4'-(4-aminobenzoyl)biphenyl-4-sulfonamide | C19 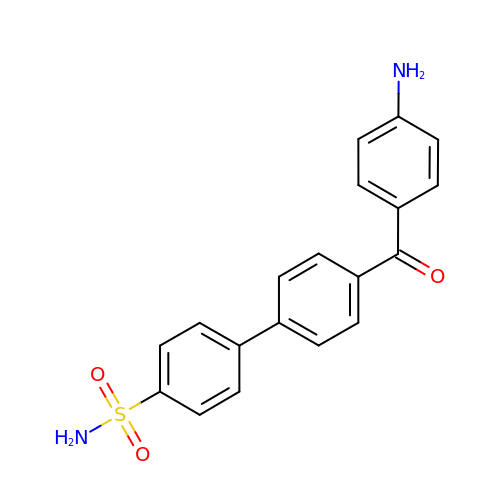H16 N2 O3 S | XKAQFZLONLOUSN-UHFFFAOYSA-N>ADCAKGKIEFSKYNEDNTFTVKVSGREYWTNRWNLQPLLQSAQLTGMTVTIISNTCSSGSGFAEVQ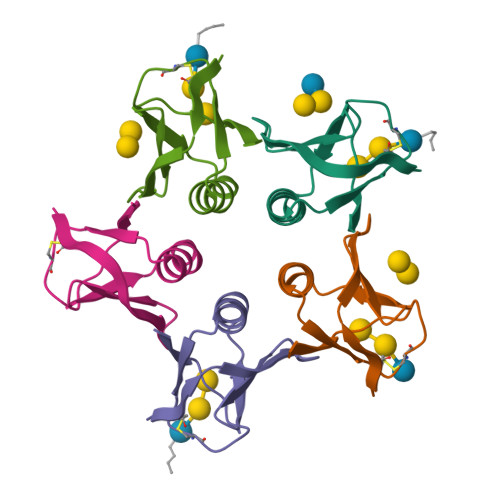FN[5x]PldA, a phospholipase D (PLD) effector, catalyzes hydrolysis of the phosphodiester bonds of glycerophospholipids—the main component of cell membranes—and assists the invasion of the opportunistic pathogen Pseudomonas aeruginosa. As a cognate immunity protein, PA3488 can inhibit the activity of PldA to avoid self-toxicity. PldA is mainly composed of 27 α-helices, 25 β-strands, twelve 310 helices, and many loops, folding into three regions: the core catalytic domain (CCD, aa 24–935), the peripheral helical domain (PD, aa 215–441 + aa 647–721), and a small C-terminal domain (CTD, aa 936–1094). Compared to the open conformation exhibited by PldAFL (pre-open state), PldAtruncate presents a highly open conformation (open state) and the PA3488-inhibited PldA reveals an almost closed conformation (pre-closed state).

Here, we have determined, for the first time, the crystal structure of the full-length eukaryotic-like PldA (PldAFL) in the apo state. Close examination indicates that the reactive His167–His855 pair resides in the loop connecting β4–β5 of the HKD1 domain and β17–β18 of the HKD2 domain, spatially in the vicinity of catalytic Lys169 and Lys857, respectively. Moreover, the imidazole group of His855 from the HKD2 subdomain, mediated by two water molecules (W1 and W2), indirectly forms a three-hydrogen-bond network with the His167–Lys169–Asp184 pair, thus stabilizing the active site. The conformation of the active site region is almost identical to that in eukaryotic PLDs rather than prokaryotic PLDs, indicating a eukaryotic-like catalytically active PLD conformation of PldA. In PldA, the main chain carbonyl oxygen of Ile1072 forms a hydrogen bond to the side chain of Arg876 from the α24 helix, which is adjacent to the conserved HKD domain. The B factor (The scores are negatively correlated with the stability of one structure) of the PD region is extremely high, suggesting that this region is structurally dynamic; in line with this observation, molecular dynamics simulations of PldAFL showed that the positions of these helices fluctuate. In PldAFL, the α11 helix stacks against the α4 and α9 helices, and these two helices clamp the α3 helix connected to the lid region, thus stabilizing its conformation. In PldAFL, the lid region forms a short 310 helix (residues 120–122), packing with the β2-α2 loop and the α8 helix. In such case, the lid region is positioned distant from the entrance of the active-site pocket, which becomes accessible to the solvent so that the substrate can gain access. Our structures of PldAFL and the existing hPLD structures show that they adopt an “open” conformation, with the potential lid region draping away from the active site and allowing the accessibility of the active site to the solvent and the substrate.

> MLQKKPYNGLHEKELNQINQQDGSPCVAISAPGCFIKGSNLFSEKRAGNRVRFFTTGRDYFSDLASALDSASSSIFITGWQVNYDVLLDGRRSLWQCLRQALERSPALKVYVMPWLSPSGSLGTYDFETMLAVFQLNAGLEGGARAFCTPAIQQSDMQGLGVAFSHHQKSVVIDNRIGYVGGIDLAYGRRDDNDFSLDASGRRGNDAYNPGLPHLGWMAEDEHVSSMGLMMATLFDLSRPLASLTLHAPTLRLSPFPHIAASDEPLLSIPLAPSRARALNGAAYLSDLFRSPMLPSLQWLGRAYNSSKEGLDEGFERLDALRRQMVASSIRAIANLIADNLDALPIEPELERRLRAWLEELRTAALNLPEALRIKSLLLINQWMSETELGQVLTLISGKGFEDIPQNLSGKAGELAGSLFWTLHRLMQARAGGHQQPYRYLDEAPQPLASPDNARLAADQPRMPWQDVHCRIEGPSVYDLARNFIDRWNGQQAYLAKTPALQDTALVRSALEAVMKWLNSLAAAAGLENYLDEKRNLRLELDPPTPCWINAPEQLPQEPEVRRGGMTVQVLRSAAARMLEQEQAGRLGAGVNLPLQVGVSTEGVQSNCKDAMLLAISGAQQFIYIENQFFQSEFGKEGEVFKDLPLSGPMASLRDVGSLRRDFVVRIRLEEALEQRDLWLLDWAEVEKIAQEPGTEARQFLKSMLAMWGVNAQGWLTHKLGEAQHGLLNEIGEALARRIERAIQREHPFHVYLVLPVHPEGALNVPNIMHQVHLTQQSLVFGEQSLVKRIQRQMALKALEGKSDPAQAREIIERKDARGRPVYEQQDWSRYLTLLNLRTWAVLGGRVVTEQIYVHSKLLIADDRVAILGSANINDRSLQGERDSELAVMVRDSEPLTVRLDGKNDAIVGKAIHQLRVNLWKKHFGLSQGPGGFVKPASELSAYLSIPAAQEAWEAIQTLAKENTRAYERTFNFIPQNISQTQLQLTPEPPKGFEDGFPASIWPTWAYRKPGELRAGGQLMEPMPYQEIFWRSSNLTSVKTFPPPNGVSGFITALPTSWTRGERNDSGLNLSILAHQDSRSLPTQVAMNGDSSAQGKHRT>VFHKIRNEDLIFNESLGQGTFTKIFKGVRREVGDYGQLHETEVLLKVLDKAHRNYSESFFEAASMMSKLSHKHLVLNYGVCFCGDENILVQEFVKFGSLDTYLKKNKNCINILWKLEVAKQLAWAMHFLEENTLIHGNVCAKNILLIREEDRKTGNPPFIKLSDPGISITVLPKDILQERIPWVPPECIENPKNLNLATDKWSFGTTLWEICSGGDKPLSALDSQRKLQFYEDRHQLPAPKAAELANLINNCMDYEPDHRPSFRAIIRDLNSLFT[2x]

JAK2 protein contains seven homology domains (JH1-7), of which JH1 (residues 836-1132) is the kinase domain, and JH2 (residues 543-824) is the pseudokinase domain. The JH2 domain has no catalytic activity but could negatively regulate the activity of JH1 and inhibit the kinase activity of JAK2. The V617F mutation site is located above the N-terminus of the JH2 domain, and when the valine at position 617 is replaced by phenylalanine with a higher molecular weight, the prolongation of helix C and the interaction between F617 and the helix C phenylalanines 594 and 595 of JH2 domain is stable and activates the JH1 domain. Janus kinase 2 (JAK2) hyperactivation by JAK2V617F mutation leads to myeloproliferative neoplasms (MPNs) and targeting JAK2 could serve as a promising therapeutic strategy for MPNs.

Here, we report that Flonoltinib Maleate (FM), a selective JAK2/FLT3 inhibitor, shows high selectivity for JAK2 over the JAK family. The results showed that FM could bind JAK2 JH2 and JAK2 JH2V617F protein with the KD values of 3.14 and 5.21 µM, respectively, indicating that FM had a better affinity for JAK2 JH2 compared to JAK2 JH1 and JAK2 JH2V617F. We obtained the crystal structure of the complex of JAK2 JH2 and FM. Two nitrogen atoms of pyrimidine-2-amine in FM were found to form two hydrogen bonds with the carbonyl and NH backbone of V629 in the hinge region of JAK2. The hydrophobic interaction between FM and the surrounding amino acid residues of JAK2 could also be found in the complex of JAK2 JH2 and FM. The L551, I559, L579, and L680 of JAK2 could further enhance the binding stability between FM and JAK2 JH2. The benzene of FM could form a hydrophobic interaction with the side chain of L551. The I559 of JAK2 also interacted with the pyrazole ring of FM with hydrophobic interaction. In addition, the other hydrophobic residues near the active binding site also contributed to the binding affinity, such as the V610, F628, and F631 for JAK2. However, FM is different from previous JAK2 inhibitors because of its unique ability to selectively bind to the JH2 domain of JAK2, exerting its function through an allosteric mechanism.> G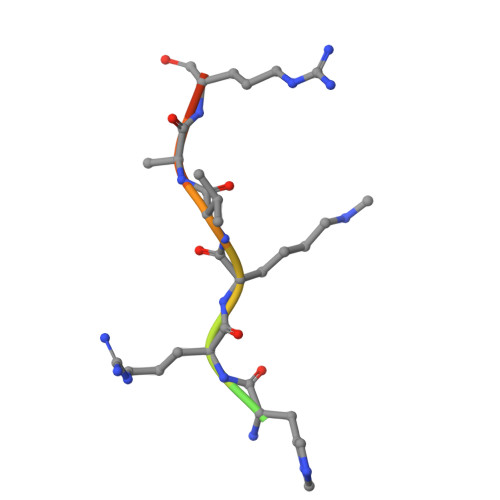AKRHRKVLRDN>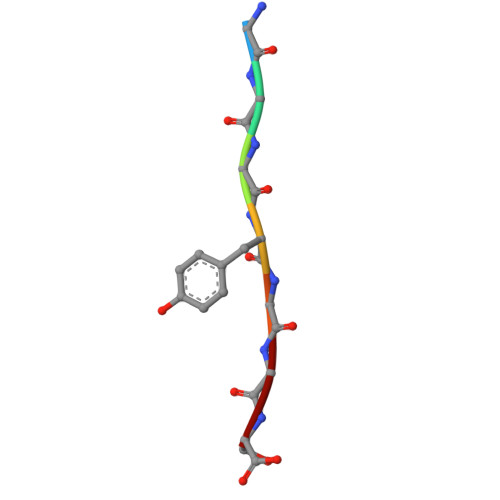[2x]GGGYGGS> MV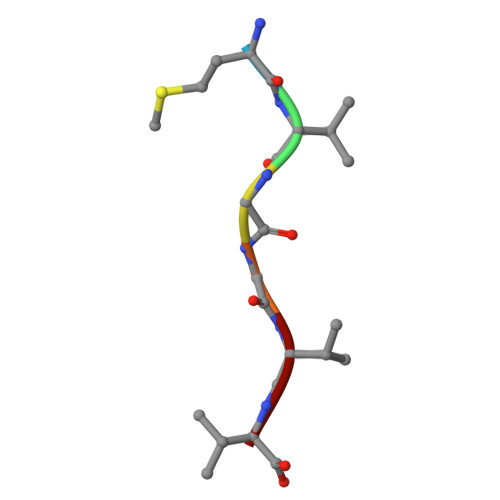GGVV> MSLLNIKFTDNAVDYLKRREILDKILILITDDGGGKYSIQGGS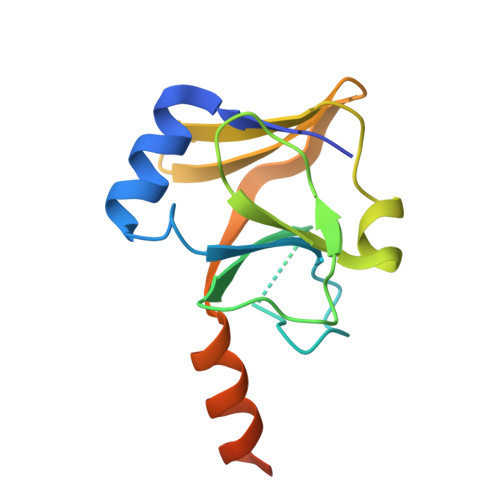CSMGAHFSIIWLDKVDPDYPVKIANEQNVKIYTSDFDKTMLGPNMVMDYNAGSLSLSSDEGLLDGSVDIGNGAALLKANKNVQMGINRQCEGHHHHHH> RLTVVKQYVDNVLNKASDTYHGD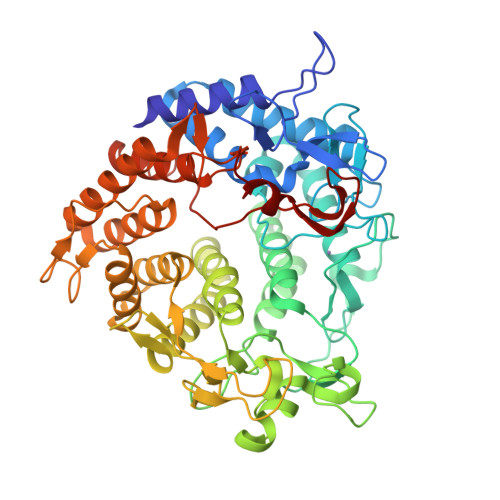KPSPLLADGVDPRTGQQLEWIFPDGRRAVLSNFSAQQNLMRVMSGLSQLSGDPRYQKRAEDIVRYHFQNYQDPSGLLYWGGHRFVDLKTLQPEGPSEKEMVHELKNAYPYYDLMFSVDSDATARFIRGFWNAHVYDWRILETSRHGEYGKPMGALWESKFEQQPPFFATKGLSFLNAGNDLIYSASLLYKHQQDQGALTWAKRLADQYVLPRDAKTGLGVYQFTQALKREEPTDDADTHSKFGDRAQRQFGPEFGPTALEGNMMLKGRTSTLYSENALMQLQLGKDLGPQGQDLLKWTVDGLKAFAKYAYNDQDNTFRPMIANGQDLSNYTLPRDGYYGKKGTVLKPYKAGNEFLISYARAYAIDNDPLLWKVARGIANDQGLGDIGTAPGKEVKVNMDTTNSDPYALFALLDLYHASQVADYRKLAEKIGDNIIKIRYIDGFFMASSDRQYADVDAIEPYALLALEASLRNKPQAVAPFLNGAGFTEGAYRMDDGSARVSTRDNELFLLNV DIHYDROGENPHOSPHATE ION | H2 O4 P | 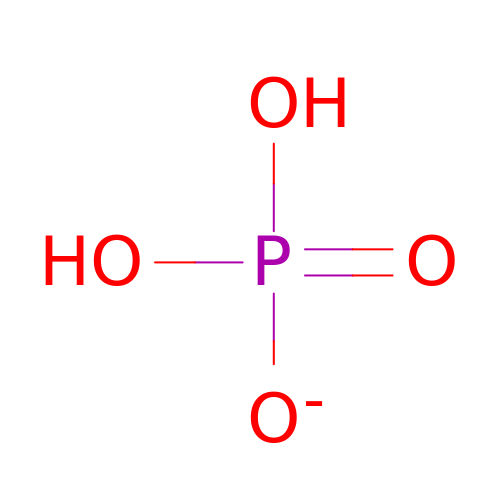NBIIXXVUZAFLBC-UHFFFAOYSA-M Ivabradine 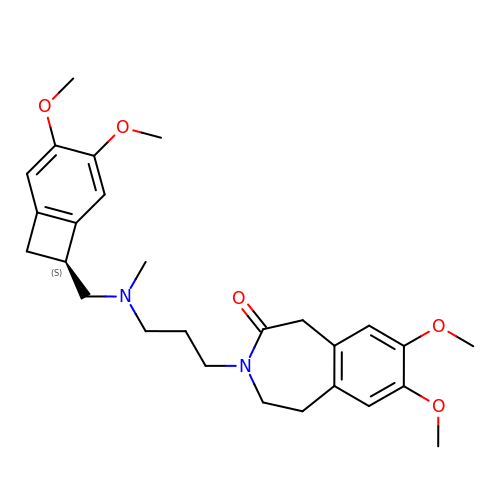| C27 H36 N2 O5 | ACRHBAYQBXXRTO-OAQYLSRUSA-N methyl (2R)-3-(furan-2-yl)-2-(pyridin-4-yl)propanoate | C13 H13 N O3 | 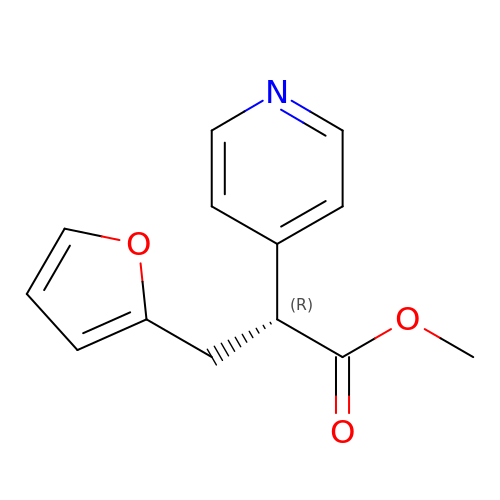DTRVWRJNHJVAQQ-GFCCVEGCSA-N>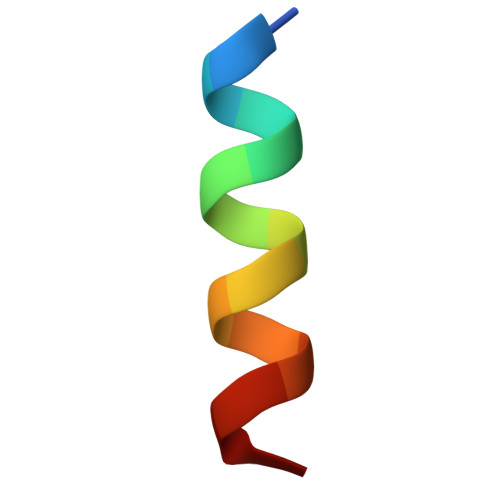 GSLLRVQAHIRKKMV> GSRRASVGSHEVEKSGLLNMTKIAQGGRKLRKNWGPSWVVLTGNSLVFYR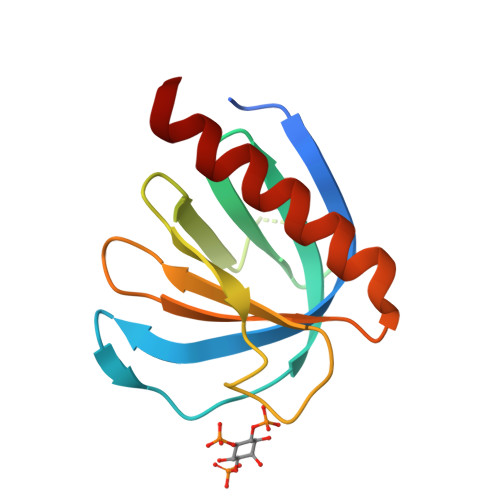EPPPTAPSSGWGPAGSRPESSVDLRGAALAHGRHLSSRRNVLHIRTIPGHEFLLQSDHETELRAWHRALRTVIERLVRW> GPMGSAQLLKSVFVKNVGWATQLTSGAVWVQFNDGSQLVVQAGVSSISYTSPNGQTTRYGENEKLPDYIKQKLQCLSSILLMFSNP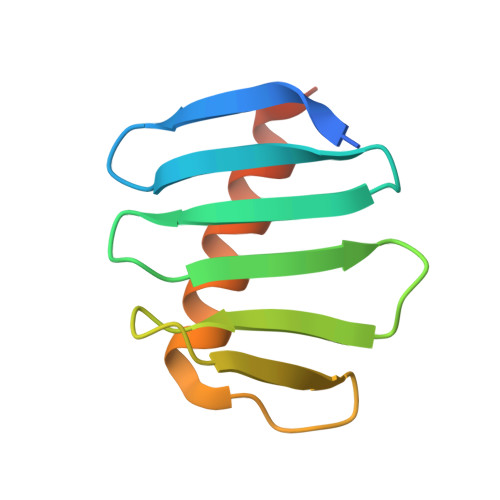TPNFH> SSESIRMVLIGPPGAGKGTQAPNLQERFHAAHLATGDMLRSQIAKGTQLGLEAKKIMDQGGLVSDDIMVNMIKDELTNNPACKNGFILDGFPRTIPQAEKLDQMLKEQGTPLEKAIELKVDDELLVARITGRLIHPASGRSYHKIFNPPKEDMKDDVTGEALVQRSDDNADALKKRLAAYHAQTEPIVDFYKKTGIWAGVDASQPPATVW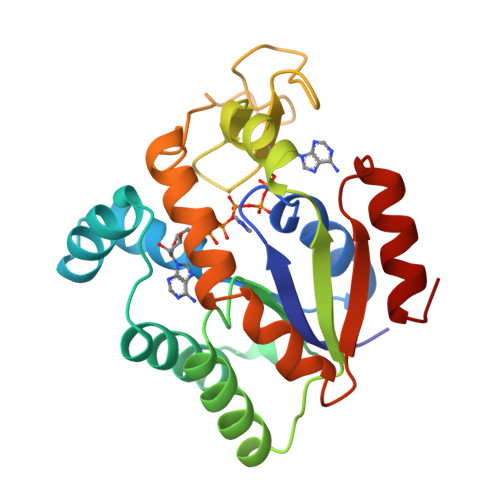ADFLNKLGKN> GPMVALSLKISIGNVVKTMQFEPSTMVYDACRMIRERIPEALAGPPNDFGLFLSDDDPKKGIWLEAGKALDYYMLRNGDTMEYRKKQRPLKIRMLDGTVKTIMVDDSKTVTDMLMTICARIGITNHDEYSLVRELMEEKKDELNWLDHGRTLREQGVEEHETLLLRRKFFYSDQNVDSRDPVQLNLLYVQARDDILNGSHPVSFDKACEFAGFQCQIQFGPHNEQKHKAGFLDLKDFLPKEYVKQKGERKIFQAHKNCGQMSEIEAKVRYVKLARSLKTYGVSFFLVKEKMKGKNKLVPRLLGITKECVMRVDEKTKEVIQEWSLTNIKRW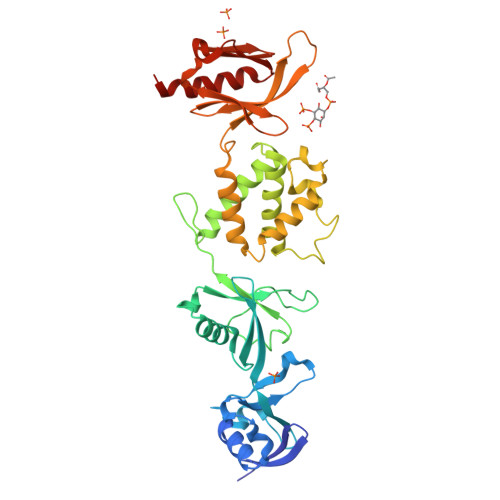AASPKSFTLDFGDYQDGYYSVQTTEGEQIAQLIAGYIDIIL EPCR is a transmembrane MHC class I-like glycoprotein primarily abundant in the vasculature of large vessels, but present in numerous cell types. Since its identification, EPCR has been mainly known for its role in accelerating the generation of the anticoagulant activated protein C (APC) and favoring its cytoprotective properties. Structurally, EPCR shares a notable degree of homology with the CD1 family of receptors, including the presence of a central and extended hydrophobic cavity suitable for lipid antigens, flanked by two alpha helices lying on top of a beta sheet. The presence of a lipid bound to EPCR is key for its biological functions.

For this, we performed a wide crystallization screen and obtained EPCR crystals in varied conditions, which ultimately led to solution of the structure in three different space groups. Crystals grown in other conditions yielded EPCR structures in two novel space groups, C2221 and P212121, containing 2 and 4 molecules of EPCR per asymmetric unit, respectively. Structural alignment against EPCR in space group P3121 yielded root mean square deviations of 0.459 and 0.400 for EPCR molecules in space groups C2221 and P212121. We observed, however, non-homogeneous signals inside the lipid cavities. Fitting of a diacyl phospholipid scaffold (lacking the outermost head group) satisfied the overall shape of the map, albeit with some degree of uncertainty for the orientation of the carbonyl groups. Despite the high resolution, we observed a less accurate electron density map in one of the two EPCR molecules in space group C2221, where the signal appears disconnected and fitting of a diacyl phospholipid results less satisfactory. The only molecule found in P3121 yield a ~ 1375 Å3 cavity while the two molecules in the asymmetric unit of C2221 have pockets of 1410 and 1540 Å3.

>GPSQDASDGLQRLHMLQISYFRDPYHVWYQGNASLGGHLTHVLEGPDTNTTIIQLQPLQEPESWARTQSGLQSYLLQFHGLVRLVHQERTLAFPLTIRCFLGCELPPEGSRAHVFFEVAVNGSSFVSFRPERALWQADTQVTSGVVTFTLQQLNAYNRTRYELREFLEDTCVQYVQKHISAENTKGSQTSRSYTS[2x]>MKKRDDLTKDTPEVSEGGLSRRRFMGAAALAGVAGATGLGTSVMSRETWAAAAEEARNKAHVAPGELDEYYGFWSGGHQGEVRVLGVPSMRELMRIPVFNVDSATGWGITNESKEILGGDQQYLNGDCHHPHISMTDGRYDGKYLFINDKANTRVARIRLDIMKTDKITHIPNVQAIHGLRLQKVPKTNYVFCNAEFVIPQPNDGTDFSLDNSYTMFTAIDAETMDVAWQVIVDGNLDNTDADYTGKYAASTCYNSERAVDLAGTMRNDRDWVVVFNVERIAAAVKAGNFKTIGDSKVPVVDGRGESEFTRYIPVPKNPHGLNTSPDGKYFIANGKLSPTVSVIAIDKLDDLFEDKIELRDTIVAEPELGLGPLHTTFDGRGNAYTTLFIDSQVCKWNIADAIKHYNGDRVNYIRQKLDVQYQPGHNHASLTESRDADGKWLVVLSKFSKDRFLPVGPLHPENDQLIDISGEEMKLVHDGPTYAEPHDCILVRRDQIKTKKIYERNDPYFASCRAQAEKDGVTLESDNKVIRDGNKVRVYMTSVAPQYGMTEFKVKEGDEVTVYITNLDMVEDVTHGFCMVNHGVSMEISPQQTASVTFTAGKPGVYWYYCNWFCHALHMEMGGRMLVEKA[4x]

Copper-containing nitrous oxide reductase catalyzes a 2-electron reduction of the green-house gas N2O to yield N2. It contains two metal centers, the binuclear electron transfer site CuA, and the unique, tetranuclear CuZ center that is the site of substrate binding. MnN2OR forms the typical head-to-tail homodimer, with the N-terminal, seven-bladed β-propeller domain of one monomer in close contact with the C-terminal cupredoxin domain of the other. At the interface of both domains, the CuA site closely approaches the CuZ cluster of the other subunit to form a combined active site that is accessible via a hydrophobic substrate channel running along the subunit interface, with a water-filled cavity behind the CuZ cluster.

Hypothesizing that many reported discrepancies in the structural data may be due to radiation damage during data collection, we determined the structure of anoxically isolated Marinobacter nauticus N2OR from diffraction data obtained with low-intensity X-rays from an in-house rotating anode generator and an image plate detector. Diffraction data from a plate-like single crystal of MnN2OR were collected using Cu Kα radiation (λ = 1.5418 Å) on a rotating anode X-ray generator with a mar345dtb image plate detector at a temperature of 100 K. The crystal belonged to the triclinic space group P1 and diffracted beyond the detector edge at the minimal possible crystal-to-detector distance, yielding data to 1.5 Å resolution with a mean I/σ(I) of 2.6 in the highest resolution shell. The two N2OR dimers of the asymmetric unit indeed differed in the conformation of residue H579, which was a ligand to CuA1 in the A protomer of both dimers (IN conformation), but rotated toward S546 in protomer B (OUT-conformation). While the environment of CuA2 changed only with respect to C618, the missing H579 now caused CuA1 to move almost fully into the plane of C614, C618, and M625, so that the coordination geometry became trigonal planar, while the environment of CuA2 remained trigonal pyramidal. Contrary to the IN- and OUT-conformations of the CuA sites, the four individual observations of CuZ were indistinguishable in the low-dose structure, where CuZ consistently was a [4Cu: 2S] site, with a largely symmetric Cu2S2 diamond core that is reminiscent of CuA. In the present analysis of MnN2OR, the Ca2+ site was fully defined and showed a typical coordination environment that in essence was octahedral but included two bidentate ligands, E260 and D274. The second ion-binding site in N2OR thus holds a K+ ion that plays a very specific role in connecting the CuA and CuZ sites, integrating them into a single functional active site within N2OR. Our analysis of the anomalous scattering properties of all ion sites supports an assignment as Cl– rather than S2–, but its influence on the properties of CuZ—if any—remains to be understood.>LGTLPAFLPCELKPHGLVDCNWLFLKSVPRFSAAASCSNITRLSLISNRIHHLHNSDFVHLSNLRQLNLKWNCPPTGLSPLHFSCHMTIEPRTFLAMRTLEELNLSYNGITTVPRLPSSLVNLSLSHTNILVLDANSLAGLYSLRVLFMDGNCYYKNPCTGAVKVTPGALLGLSNLTHLSLKYNNLTKVPRQLPPSLEYLLVSYNLIVKLGPEDLANLTSLRVLDVGGNCRRCDHAPNPCIECGQKSLHLHPETFHHLSHLEGLVLKDSSLHTLNSSWFQGLVNMSVLDLSENFLYESIQHTNAFQNLTRLRKLNLSFNYRKKVSFARLHLASSFKNLVSLQELNMNGIFFRSLNKYTLRWLADLPKLHTLHLQMNFINQAQLSIFGTFRALRFVDLSDNRISGPSTLSEATPEEADDAEQEELLSADPHPAPLSTPASKNFMDRCKNFKFTMDLSRNNLVTIKPEMFVQLSRLQCLSLSHNSIAQAVQGSQFLPLTNLQVLDLSHNKLDLYHWKSFSELPQLQALDLSYNSQPFSMKGIGHNFSFVAHLSMLHSLSLAHNDIHTRVSSHLNSNSVRFLDFSGNGMGRMWDEGGLYLHFFQGLSGLLKLDLSQNNLHILRPQNLDNLPKSLKLLSLRDNYLSFFQWTSLSFLPNLEVLDLAGNQLKALTNGTLPNGTLLQKLDVSSN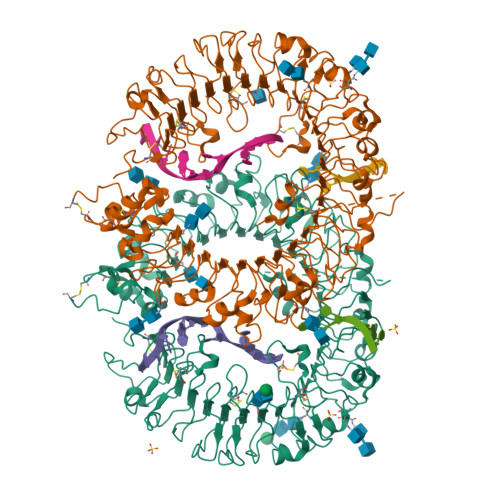SIVSVVPAFFALAVELKEVNLSHNILKTVDRSWFGPIVMNLTVLDVRSNPLHCACGAAFVDLLLEVQTKVPGLANGVKCGSPGQLQGRSIFAQDLRLCLDEVLSWD[2x]> MKIDRMRVFMTRDKDRPRVIVALDTDDGLTGWGECYNHGPDKALPPILDYLYGFLSGQDPTRIDYLVNLLIQQSRFPPGALGLSAISALDHCLWDLSAKAANVPVYKLLGGAVRDRVKVYAGVYTAPDAPAARDEFDRLNAEWGFTAFKLSPWRVDIHAHRWGNVVKASADYFRSLRETVRDDYEIAFD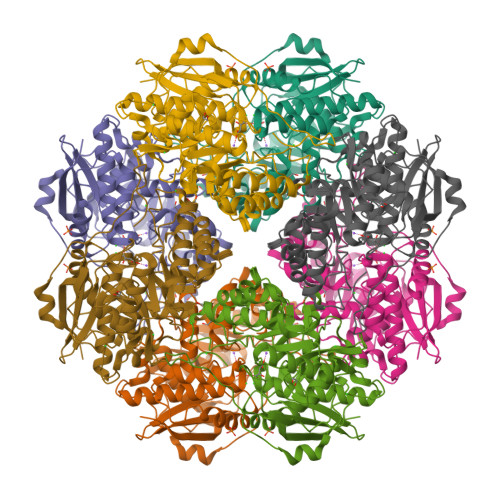AHAQIFEPVAARQLGNALAPYDPLFYEEPLRPENIDMWGDLKQGLNCVLATGESLYNRNEFLRLLQVKGADLIQPDICVVGGISEMRRIATLAEAYFVGVAPHNPMGPLATAVNVHFSAATQNFRILEYRLPKGQAYVYGGKDIEKRQGETRYVVDPYLPKDGYLELRPDRPGWGVEMDEKAMEEEGYIHWQRRVPKRPDGSYAFA5'-O-[N-(L-GLUTAMINYL)-SULFAMOYL]ADENOSINE 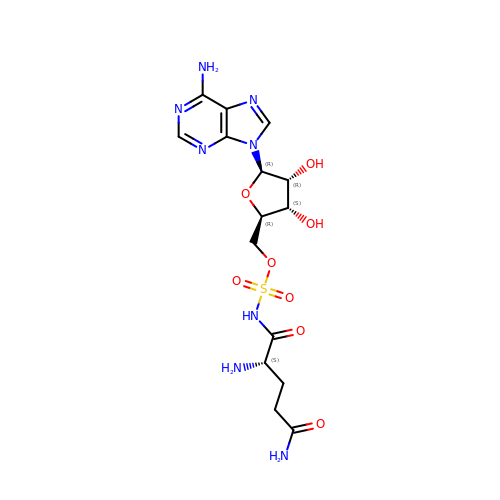| C15 H22 N8 O8 S | KXWKSWRGZLZHEF-WERHYGNASA-N1-[(2-HYDROXYLPHENYL)AMINO]3-GLYCEROLPHOSPHATE 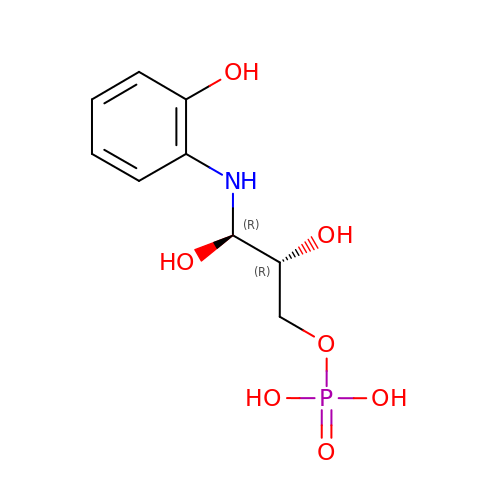| C9 H14 N O7 P | SPOVITMZOKMJPQ-RKDXNWHRSA-N> KKATQAS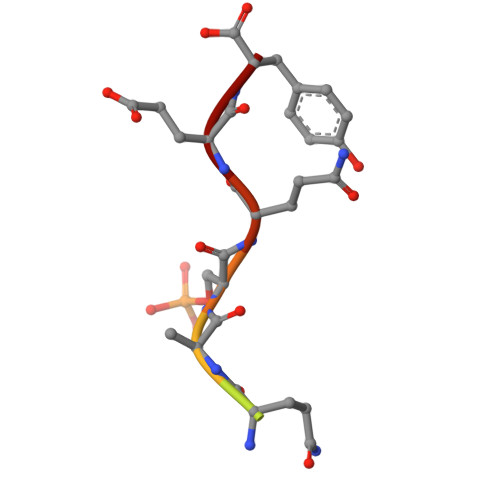QEY> MTALTPDLTTATPRLQYFHIAGPGTREYLSEDLQQFISATGSYFDLKNKFRQTVVAPTRNVTTEKAQRLQIRFYPIQTDDTPNSYRVRYSVNVGDSWVLDMGATYFDIKGVLDRGPSFKPYGGTAYNPLAPREAIFNTWVESTGPQTNVVGQMTNVYTNQTRNDKTATLQQVNSISGVVPNVNLGPGLSQLASRADVDNIGVVGRFAKVDSAGVKQAYGAYVKPVKDDGSQSLNQTAYWLMDNGGTNYLGALAVEDYTQTLSYPDTVLVTPPTAYQQVNSGTMRACRPNYIGFRDNFINLLYHDSGVCSGTLNSERSGMNVVVELQDRNTELSYQYMLADMMSRHHYFALWNQAVDQYDHDVRVFNNDGYEEGVPTYAFLPDGHGAGEDNGPDLSNVKIYTNGQQDKGNVVAGTVSTQLNFGTIPSYEIDIAAATRRNFIMSNIADYLPDKYKFSIRGFDPVTDNIDPTTYFYMNRRVPLTNVVDLFTNIGARWSVDQMDNVNPFNHHRNWGLKYRSQLLG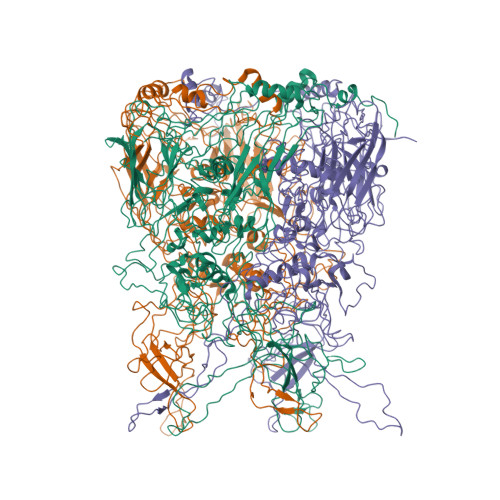NSRYCRFHIQVPQKYFAIKNLLLLPGTYTYEWVLRKDPNMILQSSLGNDLRADGAQIVYTEVNLMANFMPMDHNTSNQLELMLRNATNDQTFADYLGAKNALYNVPAGSTLLTINIPARTWEGMRGWSFTRLKASETPQLGAQYDVGFKYSGSIPYSDGTFYLSHTFRSMSVLFDTSINWPGNDRLLTPNLFEIKRPVATDSEGFTMSQCDMTKDWFLVQMATNYNYVYNGYRFWPDRHYFHYDFLRNFDPMSRQGPNFLDTTLYDLVSSTPVVNDTGSQPSQDNVRNNSGFIAPRSWPVWTAQQGEAWPANWPYPLIGNDAISSNQTVNYKKFLCDNYLWTVPFSSDFMYMGELTDLGQNPMYTNNSHSMVINFELDPMDENTYVYMLYGVFDTVRVNQPERNVLAMAYFRTPFATGNAV>QVTTEAPAKVVKHSKKQDENIVVNKFKPKE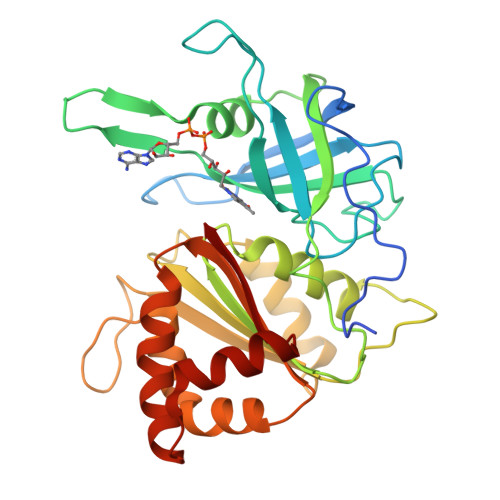PYVGRCLLNTKITGDDAPGETWHMVFSTEGEVPYREGQSIGIVPDGIDKNGKPHKLRLYSIASSAIGDFGDSKTVSLCVKRLVYTNDAGEVVKGVCSNFLCDLKPGSEVKITGPVGKEMLMPKDPNATVIMLGTGTGIAPFRSFLWKMFFEKHEDYQFNGLAWLFLGVPTSSSLLYKEEFEKMKEKAPENFRLDFAVSREQVNDKGEKMYIQTRMAQYAEELWELLKKDNTFVYMCGVKGMEKGIDDIMVSLAAKDGIDWIEYKRTLKKAEQWNVEVY[2x]((2R,3S,4S,5S)-3,4-DIHYDROXY-5-(HYDROXYMETHYL)-5-((2R,3S,4S,5S,6R)-3,4,5-TRIHYDROXY-6-METHOXY-TETRAHYDRO-2H-PYRAN-2-YLOXY)-TETRAHYDROFURAN-2-YL)METHYL 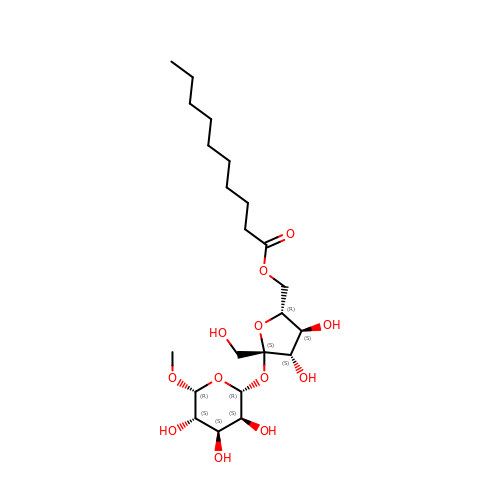NONANOATE | C22 H40 O12 | GCKKEFVHVGTJPT-PZOSHJPSSA-N>MNGGHIQLIIGPMFSGKSTELIRRVRRYQIAQYKCVTIKYSNDNRYGTGLWTHDKNNFEALEATKLCDVLQSITDFSVIGIDEGQFFPDIVEFCERMANEGKIVIVAALDGTFQRKPFNNILNLLILSEMVV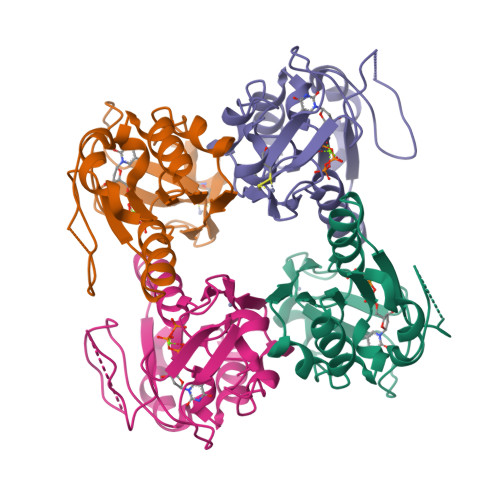KLTAVCMKCFKEASFSKRLGEETEIEIIGGNDMYQSVCRKCYVGS[4x]> KQAAQSTFNSFHEWAKQAEAMRNPSRMDIYKIYKQDAPHSHPM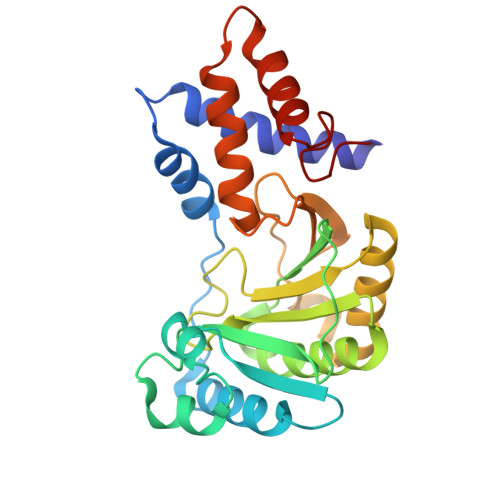SDEQQEEFLHTLKALNGKNGIEVRTQDHDSVRNKKDRNLDKYIAESPDAKRFFYRIIPKHERREDKNQGRLTIGVQPQYATQLTRAMATLIGKESAITHGKVIGPACHGQMTDSAVLYINGDVAKAEKLGEKLKQMSGIPLDAFVEHTPLSMQSLSKGLSYAESILGDTRGHGMSRAEVISDALRMDGMPFLARLKLSLSANGYDPDNPALRNT4-[(4-{[2-(trifluoromethoxy)phenyl]amino}pyrimidin-2-yl)amino]benzoic 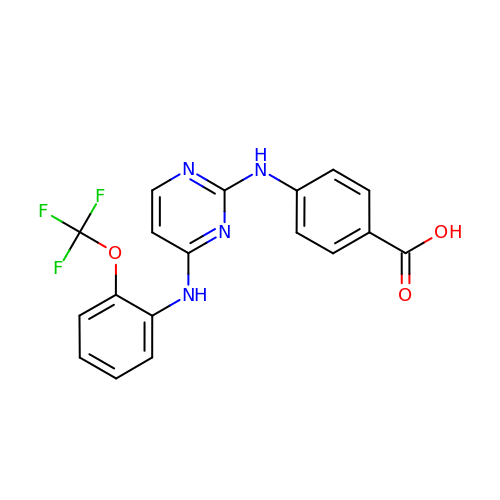acid | C18 H13 F3 N4 O3 | VKIURNGMKFWIQX-UHFFFAOYSA-N> GRRVVCERHRVVVSYPPQSEAELELKEGDIV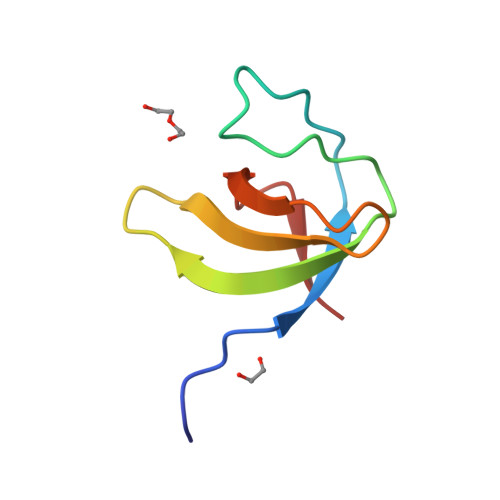FVHKKREDGWFKGTLQRNGKTGLFPGSFVENI>MPKHEFSVDMTCGGCAEAVSRVLNKLGGVKYDIDL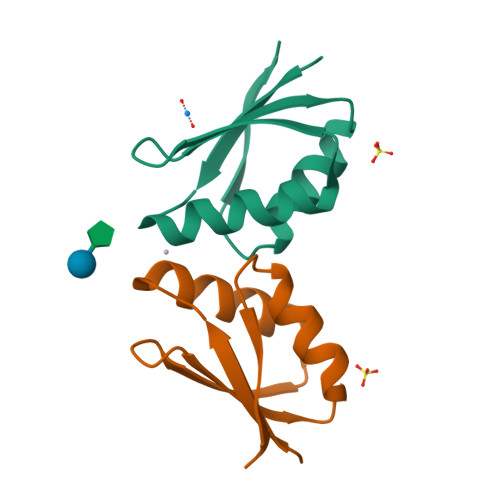PNKKVCIESEHSMDTLLATLKKTGKTVSYLGLE[2x]methyl 3-chloro-5-[(4,6-difluoro[1,1'-biphenyl]-3-yl)sulfamoyl]-4-hydroxybenzoate 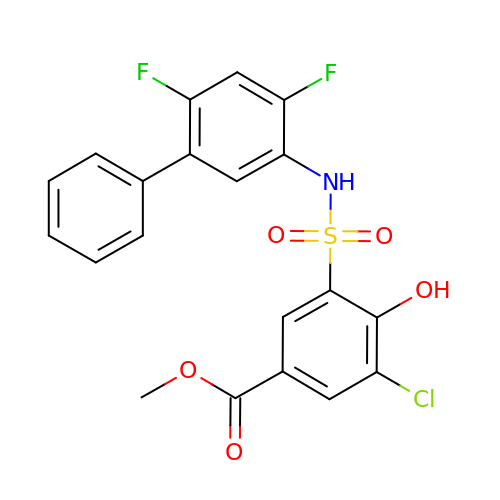| C20 H14 Cl F2 N O5 S | YSTSHUWHIDBZAK-UHFFFAOYSA-N>[2x]VDSVYRTRSLGVAAEGIPDQYADGEAARVWQLYIGDTRSRTAEYKAWLLGLLRQHGCHRVLDVACGTGVDSIML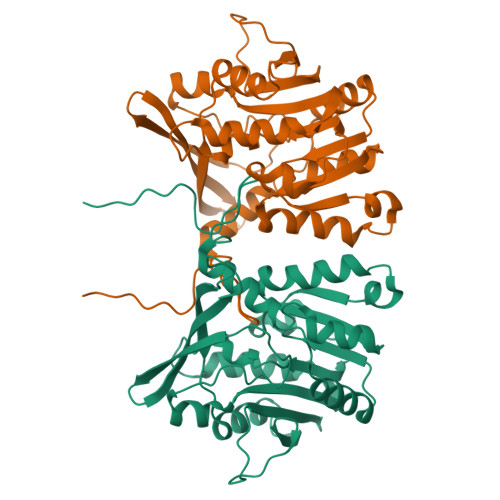VEEGFSVTSVDASDKMLKYALKERWNRRKEPAFDKWVIEEANWLTLDKDVPAGDGFDAVICLGNSFAHLPDSKGDQSEHRLALKNIASMVRPGGLLVIDHKNYDYILSTGCAPPGKNIYYKSDLTKDITTSVLTVNNKAHMVTLDYTVQVPGAGRDGAPGFSKFRLSYYPHCLASFTELVQEAFGGRCQHSVLGDFKPYRPGQAYVPCYFIHVLKKTG> MGHMEHPSRLRSQHELARRYQQNGQVQEAVELLEQVVAIQAKTLRSEHPSRLASQHELARAYMANGQVQEAVELLEQVVAIQAKTLRSEHPS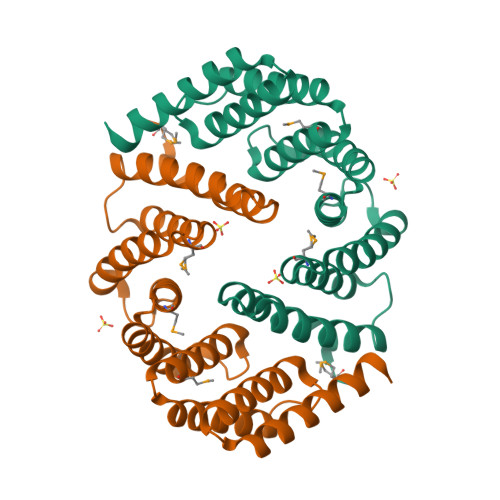RLASQHELARAYMANGQVQEAVELLEQVVAIQAKTLRSEHPSRLASQHELARAYMANGQVQEAVELLEQVVAIQAKTLRSEHPSRLASQHELARAYQANGQRQEAQELLEQVRAIQAKTQRSLVPRGSGSSHHHHHH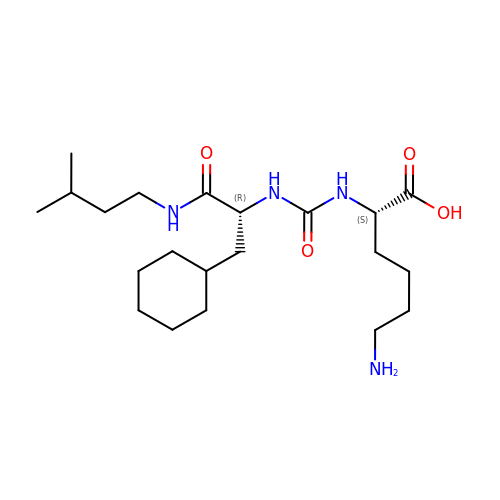(2S)-6-azanyl-2-[[(2R)-3-cyclohexyl-1-(3-methylbutylamino)-1-oxidanylidene-propan-2-yl]carbamoylamino]hexanoic acid | C21 H40 N4 O4 | PNONBGCPQRQQBB-ZWKOTPCHSA-N>GSHMGEKRSIAIDSYQEDPSVVVSNFFKGVRVPKDTEFQLYKKRKQDQFVLHGENERLEYDGETDELTTKTNQYMVGLYDKQSGKINLYRAPVVTSKIVSKF[8x];>[8x]MGMGYQPPSDYKQCKHLKSFPVSELKGDNKELWLMKVPANIDISQLKSLPLDTDATVSTVELGSKNFNVLQNTSTQEGSDNTNLSLLIPSEKKKETLKVATSKDNKSVYFDRVFT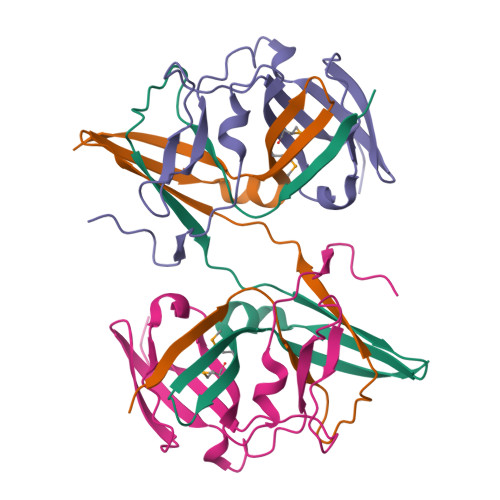ISETARIP>[2x]SCPDACCPHGSSGLRCTRDGALDSLHHLPGAENLTELYIENQQHLQHLELRDLRGLGELRNLTIVKSGLRFVAPDAFHFTPRLSRLNLSFNALESLSWKTVQGLSLQELVLSGNPLHCSCALRWLQRWEEEGLGGVPEQKLQCHGQGPLAHMPNASCGVPTLKVQVPNASVDV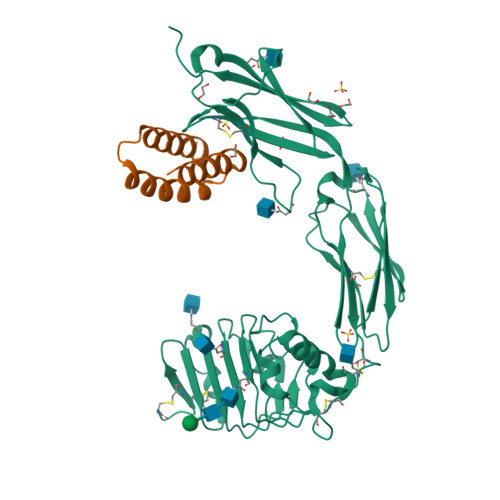GDDVLLRCQVEGRGLEQAGWILTELEQSATVMKSGGLPSLGLTLANVTSDLNRKNLTCWAENDVGRAEVSVQVNVSFPASVQLHTAVEMHHWCIPFSVDGQPAPSLRWLFNGSVLNETSFIFTEFLEPAANETVRHGCLRLNQPTHVNNGNYTLLAANPFGQASASIMAAFMDNPAAAHHHHHHHH;>[2x]MSHHHHHHHHSENLYFQSGGGRDEIKERIFKAVVRAIVTGNPEQLKEAKKLLEKLKKLGRLDQDAKKFEKAIRQVEKRLRS> MRRTVVQRVAPWVPPPRHDIKVTMPPPPGGEVGGRFGVSQGYSDRLARTPYWKRMALSTYKLRMMENATRYPMSEHRPGEYDIRYLPTPYPCTIRNRPLLEVGEPRQIPSI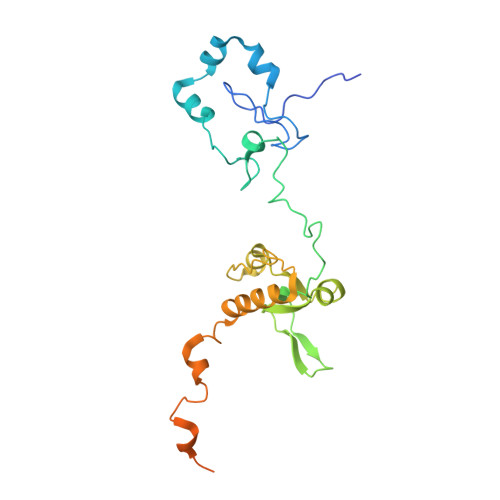RIPVIFLVNLFDEAKGCWFGRRYETVYVERQFMREELMPQRYAIYATPEAYKLLGLPVVNHHTHEEIPKTPREYEKLLERQRYDEERWKYTIEYLFRKYEDGPPELLDRPEDGWDGSEEIALSSVAGAGRDGVVSQRKGPVKQRKARKIKLF> MAAESVRVAVRCRPFNQREKDLNTTLCVGMTPNVGQVNLNAPDGAAKDFTFDGAYFMDSTGEQIYNDIVFPLVENVIEGYNGTVFAYGQTGSGKTFSMQGIETIPAQRGVIPRAFDHIFTATATTENVKFLVHCSYLEIYNEEVRDLLGADNKQKLEIKEQPDRGVYVAGLSMHVCHDVPACKELMTRGFNNRHVGATLMNKDSSRSHSIFTVYVEGMTETGSIRMGKLNLVDLAGSERQSKTGATGDRLKEATKIN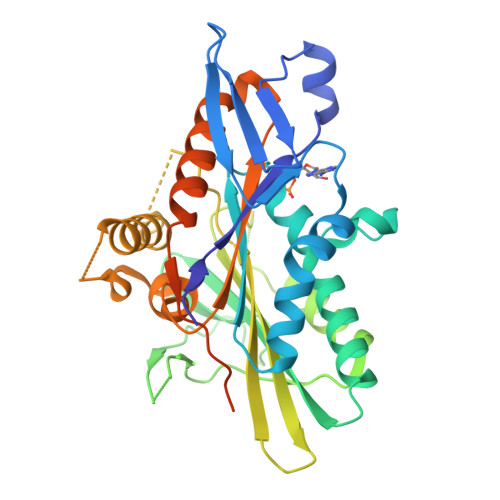LSLSALGNVISALVDGKSKHIPYRDSKLTRLLQDSLGGNTKTIMIACVSPSSDNYDETLSTLRYANRAKNIKNKPTINEDPKDALLREYQEEIARLKSMVQPGAVGPLEHHHHHH>MSGSHHHHHHSGSMSPSPIEEQATRLLKEVPLIDGHNDFPYMIRGWFRNDINGQDAHLYDMPIGQTDLQRLQKGLLGGQFWSAFVPCPKNPDKEVGSLEALRQTLQQLDVIHRLIERHPTILQFADSAASIWSSFRAGRVASLIGIEGLHQIADSVSALRMLHRLGVRYVTLTHNCHNAFADAATVSPELHGGLSRKGERLIRELNRMGMMIDLSHTSHEAQTQALRLSRAPVIYSHSSIYSLRAHARNVTDENLHLLHRNRGVVMICFLRELLASEADQATLAHVIDHIIYAGTRIGYEHVGIGSDFD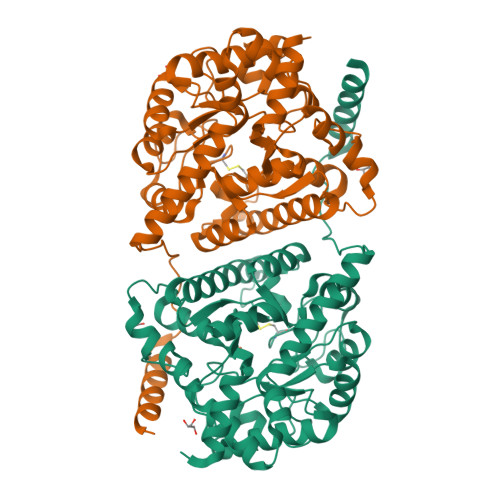GMLRGPDGLHDVSCYPALVAGLLERGVSEEDVKRVMGLNVIRVLEEVERVAAELQGAGEECLCDELDEVWNEDIKEQLTRERERVRKLGPQK[3x]>[2x]MHHHHHHRKAAGKYGNTLEFGHLVGGEEVLEGPLLERRNPSDREDVVARFPEADKDLVRKAALKAREAFAEWSRTPAPIRGQVLFNLVKILEREKPTLTRLMVREVGKTPKEAAGDVQEAIDTALFFASEGRRLYGQTVPSEMRDKELFTFRRPLGVVGIITAGNFPIAVPSWKLIPAVLTGNTVVWKPSEDAPTLSFVFAKLFEEAGLPPGVLNVVFGGGKGSTGQWMVELMDEGLFQKFAFTGSTQVGRWIGEVAGRNLIRPTLELGGKNPLVVMRDADLDLAVEGAWWSAFATGGQRCTSAGNILVDAPIYEEFKRRFLERVEATLVGNPLLHPEVTYGPFINERFFARWQEHYRVGEAEGARLLFGRGRITRENPYPRFLGDPEAGLYGWPTVWEVRPGTRLFTEEVFGPTINLVKVDGIEEAIA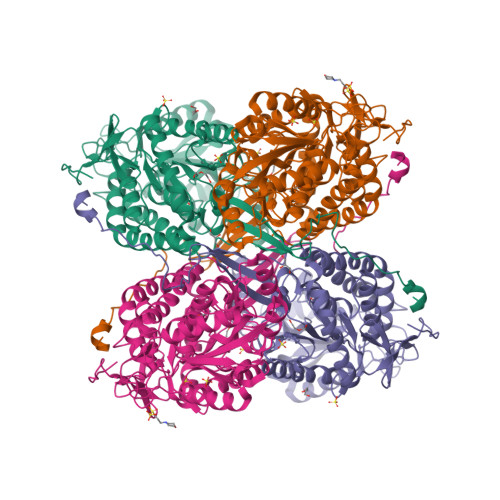VANSTPYGLSSAIYTNHRHWAYLFKVGIRAGMTSINNATVGAEAHLPFGGVKASGNGGRESGIWVLEEYTYWHAVNEEYSGRLQLAQMDTGYVSPKAPTPWGEVLGL>GMTQKEWPLWEVFV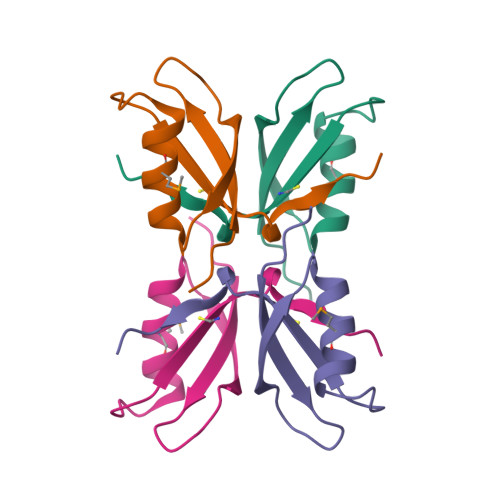RSKQGLEHKHCGSLHATDAQQALHMARDVYTRRQEGVSIWVVPSTAITASAPEEKPELFDPMADKIYRHPTFYQLPDEVNHM[2x]> MKELIIVGAGGHGNEI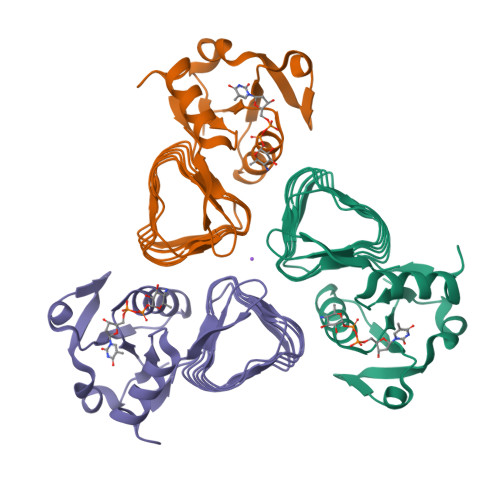SWLAKRCGRVVRGFLDNTVEKQGTFIRDIPVLGTLDECSKFTDCDFVIAIGSPRARKKIIEHFFPEGEFTFATLIDPTATIGENIHIEEGTMICAGGILTVDVKLGKHCIVNTNAVLSHGVILGDYVTVAPNASISGDVSLGNIVEIGANATIREKVSVQDGAMVGMGSVVIRNILSNQVVVGNPAKLLKVIELEHHHHHH> MDILENYVSFDEQARDINIAFDKLFGRDDISHMNNFSINKRSYYNCLDQISDDLNLVLNKYNDLAYSLLEIRYNMATKENYTHMEFYSDIERLFIKNEKLLNVISDIVEEEYDLDLNQASKGKKINIELQVTDNLNKIYLKSSVLMRILIPILCDFNCDDDINEVLVYDIFKEVIKSFDDGKKNALNKLYKIIYSRVFETKYSDVVIWTYLKNMSTDLMIIVKDYFKVIIKKIFPKLKHNSSVISYLDVVIKQKLKYLFTFKYPISYKPLKAETTDDEELSEQERMEINLLRNDQG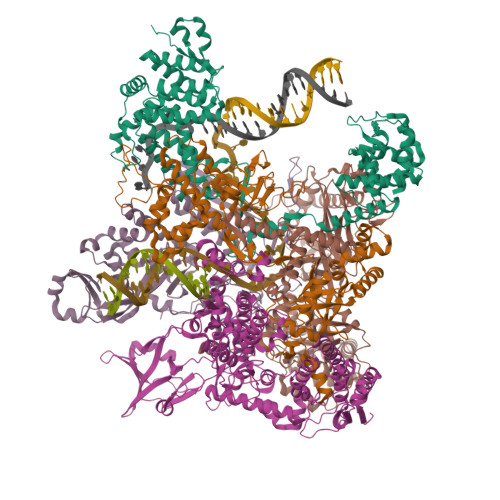NSIINECSIKQEIAKIKKKYNVTDEVMKEFINGRELNSIQIYLVKIYYSNKFKVNSNKNDIFYLLYGMTRELGEMNFSIIPEILSCAIAPNVRKMNNRKKLVDKIIHSDKYSYLLKSYLPIKNILDKNNVILQLMTIKNAKFMNKENKEVDFSTDHLAEEVLDMLLCI;> MDDISVIKNEDYEGSHRFLAEELLMPNANKTDGNRSTMFCSHLAQAVTLQKAEPPLVYTNFENQVGKYSTAGYRKANSNYKVIEKIYKNDYNYVLIVQDQETGEYTLFERAECEFLTEHYGFQWDNDKIDSLKKDDTIEKDTVLYKNTCYDENMNFGYGVNLNAAYFSYKNETLEDAIVISESAAKKLGTFSVNKVKVSVNTNDILLNLYGDNENYKGFPDIGEHIKNQIIASRRRFDYNTALYELKNLNEMRDSDTPFFADGKIVDIEIFSNVPEEELKVQKYNEQVLYYINKQKEFSNNVYQKLKKIVEGKDNNVSDKLLHFYNNCKMRIDENISYTYQNSKFSGFIMEFTILEEEPLNKGSKITGRYGNKGVISKILPDDQMPTVAEGRFKGLKADICLNPLGVFNRLNPSQLIEQELNWIAKFIRKDMEEAGSNEEKVSILLDFLNRVNKEETELMEEFINSLNKTELEEFLNDIIENGIPICQKPFFGNIGLDELWELYNHYDHIDYFKCEGISTPLIIGEIYMVRLKHEPHSKFSARSTSFMNLRGLPAKSKNFKEHKDLYSKTPVRIGNMEISNLSLTNEMGSIMDMLNSYSNNETNRRELIMQLLTGNPFDTNIDLSDVESGTSKILKSLFTCLGLSIDDVEEEWENKLNGKVEDEK;> MEKTYNLNDILLSNEYEKIKEDIKEEIINDMASKKVKYSNTSEFAKNDFLKDEFIDLVVDGETYEITYGNLITLLIVARPFNHFKVPMTEDLLFDLSDLKEYQNYYTTLLEHFGYSNEIKSIIKDVISELAIFSGDINVTFGNTVSIKSLIDLGNKVKRFRELLHYRLPNDEALEFNDIEAIIKKNLDEIMKILSETDNMLRYYIDSGAGINSKQFGQVLSLVGSKPDLFGKIIPYPINTSFLRGLDVRSFYINALGARKALITNYQQVRNSGYLTRKISMLLMDTKLIDLDDCGSHENNYLSINVENKDVLKRFSKRSYLNNNGELVEIDINDESLIGQVIKIPSPTTCASNEGVCRKCYGKLFDINKDLNIGMIAVLLLTDPLTQRLLSAKHLLETRSSKIDWGTNFEENFIVNRNLIYPKVYNGTVIIKEDDFKEDEETEEQVFDTFTLKSGNRFISISSPMRLFLNKDLKKQLDESFYNIEEMQFEIPLNKLDEGDSFATFIMDNNELSKPLREIKDLIETNKYIKDHNVNEVVNYFIYLLNESGINIQSVHSELIIREMMKLDDSDRTQFKNDKMPDYEIFRITDANLKGDSLSRSLLFEQVKKQLTTLDYDTFNKTKSSILDKLL;> MISNFRKFHGNKNQEKFNENLILNKENESILNYLDPICKTLEIIPEITYLGSSVEPINKVYKFNKEEKTSDIERSELQLIKMSFLIEKDDKKEEINKFIYFPKLIDSQYFIINGNRYYPIYQLLDSGTYRTNKALTLKTLLMPIVLREKKETFDDINGETHTMLNVDLDLFKSKVPFLIYFFSKFGFEGTLEYFGLQDLIHVLMKEDLDQLDEDEINDNVIFMITKNISLVVDKNFFSNKNNQIIIATLLNCFNTRIKIDKIYEKDYWVKKLGGYFTTNNSNKQEKGEGIILSFERILDEWTKKILRTEEKNKEDIYSVVRWMINNYLALVKQDNMNLANKRIRLYEYLLHPLLIKFSKGTYRVLNNRNSNKFEKIKTIFSNIQEGFLVKKIINNELLRYDNSVNSISLFTLILRYTQSGPQSPFSSNSTNNKLRGLHPSYLGRLGLTSTSAGDPGASGSLTPFLELPENSYMHFTEEPEINLNIDDISIDEVIES;> MGKKLSLIDFNEIYNEENLITRANPIENHEFSDDGIYSERIFGSYNEDDDDKDIDTIGWINIEPYYIINPILFTIIKKCIPSINKIINYQQSIDQNGENIDLTEEIGEDDYIGLVKFKDNFDDLLEKYTDKKKYQKEYDFLIENHDKIFINKLPVFSHKLRPATLLTGSKGKVLAFDEINNYYNFVIEYINQINEGVVSDDSIDLLLLPLLYNMQFYANNILTRIISEYLRGKKGFLRKNIMGSRINFSARNVITPLIGHPIDEVAMPYKTFAELYKFQLINLISKVKGINYNEALKFWEKGILGFNQELYNYMEELITKTKGGCTFLLNRNPTISIGSILYLKIGLIKKDYKDLTLGISNNLLSALSGDYDGDVLNIIPVFDNKMKEHFSLLSPQNFLVDRNNGRFNGDFDLQKDQILGIFILNN> GPLMSGLNDIFEAQKIEWHEGSAGGSGHMTDLRKLEALQALHAELVAVRQHRFEGLQVLETLLEEQTDAFKALIAKPARDTKDREALGKEPKKLKIGEEEYSLNEDFVNDCLKLADELDLNEKESARILIDCDAEGDVETQSRPLWECGVIRFHQERKYLLDCMRLILEIAADEDIDAGLQESFGVAAEDKIFGIPPPWERNKENQPTQVKKFIPRCMEAMKGVRSMLQCMADKANARNMLQQASLVRPLDNQETLDFSRLSLVEQHECLASILHAAVQRHHATIADFQDFIKILRKWDKYDHFLIHLIPVLAAYITEFGSPEGMGDLQQARRLNDFICKGGDEDSWALPVLGAAVRAWWIAEHNGFYLDDTVQDLRGINLDEEDEQRTKQFLDALKEGAFDFILSVAADCKAQEWQDPSQLGARQWLQRKIPSLPSEPFPFSHFLQHSLMVHLEGFVDATISNLPDVLRKLRTEEDEQRQLRPNHEQDMDLERFLIIISYAYEGRPDAAMSFWEDPDSNLAGFLQWASRRASTPLVSAFCEMLRCLADNEECATAAHNFLLDEGHQASGKMKRSQSLTWSQIFKELEYFTTKVCSERPNPPQASMHRPGRPGADPAEIEPESALMLECYLRLIAKLATESEIARKRLIMDEDFNLVDTILKLSVGVIPHRLRACIFYVLKALMIRKTHEELDAMWRWVEAWMTNPFSSLPGSQGAPQRISFLGQTPGPQECMEMMFREFGTGFEQSNAFIQLLTTLLVPPEGLNSLNDSVPFPEWLGSSIRTLGIEPYVDFVFDVFANRTKDISDPSQLRILRLSCLDFVMVCLVTFNEDLIVLGHESNISIDDAMAATNLATYVRLHPFSRVMEWLFNEKVITSLINTIHQDPISLGSASPDSPLVVSILRAIQVMIKALELQETYLHLVRPEVLRYQGEAGVRRKPVANAAYSAFEDGILSHLSLVVDLGKYCNLGHAELTLACLKLLEKISTSSRILSAWSPDSGRLGHRNKAIVQLERNGEGETISASLSASIMATLDPALAASGENYRVKLAILDFLYACLRATPDQPTIAHQLLGFH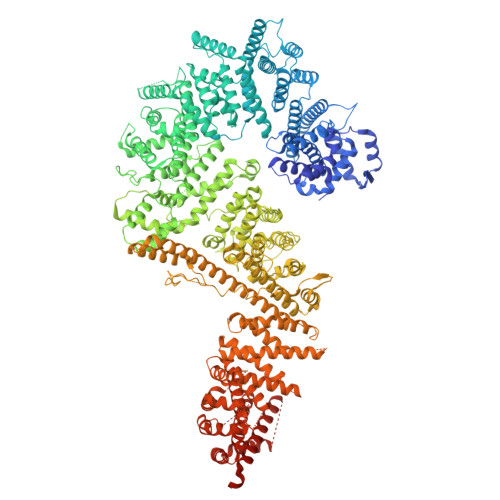CELSKLGIEPKGPFDMQKSLFHSLLNVLITLTVSEEEQGMRGYLVTLKYRVLRILQLLWKSPLSASLVMDELRATNFLFHMLLREVQIQPQLPWDGQLVTGCEFLLSDASLAYIDYLASRAAIFEYIGKELCSVSQNRIPSIKRQIFDALNGQIFVDEEAPLTIPSIFDFFDFINTDYKWEEIPSPHFTYLKDLDLGPCILEHKYAGVHYDIRKAQEILALKRKEYEHSQLATPEFLETVELEEKVLIEWLTVRNRANLLLTARLNLLQAWANLLLVMIESNDFKSTPKMAFLLQALQAILPTLEAFSSLKSDEAFELARVAKVLLWKLDFSQDSDAGLDREQFTVGNLIGDKLFQLFQLCLSAISQCSGTPELRSLYYSICYRYLTAVVDNDATVAATPASSTIGPTRSVTNARARTLKAITLYGDRLLNVICDDAYGSDTTCQTAAMILLNALVHTSRASSAAGVSPADVDCPIIDALNRLNFIGVLVDSLKEILNEWLAPSSTFDPSLSTNASPSLPIPASPSQQYTSAKLALLLQLCQTRQGAKYVLQANLFRALEQSGVFAADPELVEVDSESGVPRVVALERHYALLVALARVVGAAVTARGAHNIVQGRKFLTQHRGLVVHVLKKNAGIGGGVVGNSLASSINGGSTATMTRRDEILAQQALEERIEELAEAFMLLITATGFLEYESEQVPSEQPRAHTTFFH> MLGTGPAAATTAATTSSNVSVLQQFASGLKSRNEETRAKAAKELQHYVTMELREMSQEESTRFYDQLNHHIFELVSSSDANERKGGILAIASLIGVEGGNATRIGRFANYLRNLLPSNDPVVMEMASKAIGRLAMAGDTFTAEYVEFEVKRALEWLGADRNEGRRHAAVLVLRELAISVPTFFFQQVQPFFDNI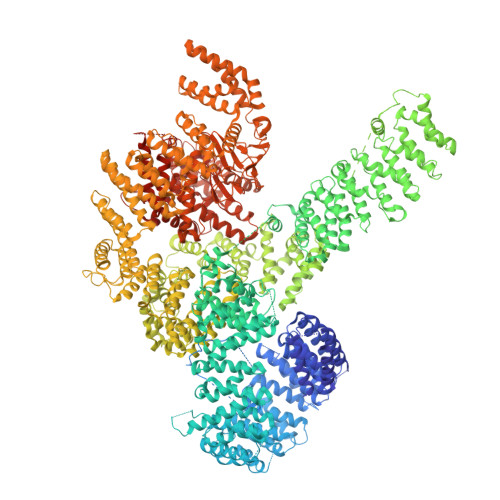FVAVWDPKQAIREGAVAALRACLILTTQREPKEMQKPQWYRHTFEEAEKGFDETLAKEKGMNRDGSTSGSGDYKDDDDKGSTSGSGDRIHGALLILNELVRISSMEGERLREEMEEITQQQLVHDKYCKDLMGFGTKPRHITPFTSFQAVQPQQSNALVGLLGYSSHQGLMGFGTSPSPAKSTLVESRCCRDLMEEKFDQVCQWVLKCRNSKNSLIQMTILNLLPRLAAFRPSAFTDTQYLQDTMNHVLSCVKKEKERTAAFQALGLLSVAVRSEFKVYLPRVLDIIRAALPPKDFAHKRQKAMQVDATVFTCISMLARAMGPGIQQDIKELLEPMLAVGLSPALTAVLYDLSRQIPQLKKDIQDGLLKMLSLVLMHKPLRHPGMPKGLAHQLASPGLTTLPEASDVGSITLALRTLGSFEFEGHSLTQFVRHCADHFLNSEHKEIRMEAARTCSRLLTPSIHLISGHAHVVSQTAVQVVADVLSKLLVVGITDPDPDIRYCVLASLDERFDAHLAQAENLQALFVALNDQVFEIRELAICTVGRLSSMNPAFVMPFLRKMLIQILTELEHSGIGRIKEQSARMLGHLVSNAPRLIRPYMEPILKALILKLKDPDPDPNPGVINNVLATIGELAQVSGLEMRKWVDELFIIIMDMLQDSSLLAKRQVALWTLGQLVASTGYVVEPYRKYPTLLEVLLNFLKTEQNQGTRREAIRVLGLLGALDPYKHKVNIGMIDQSRDASAVSLSESKSSQDSSDYSTSEMLVNMGNLPLDEFYPAVSMVALMRIFRDQSLSHHHTMVVQAITFIFKSLGLKCVQFLPQVMPTFLNVIRVCDGAIREFLFQQLGMLVSFVKSHIRPYMDEIVTLMREFWVMNTSIQSTIILLIEQIVVALGGEFKLYLPQLIPHMLRVFMHDNSPGRIVSIKLLAAIQLFGANLDDYLHLLLPPIVKLFDAPEAPLPSRKAALETVDRLTESLDFTDYASRIIHPIVRTLDQSPELRSTAMDTLSSLVFQLGKKYQIFIPMVNKVLVRHRINHQRYDVLICRIVKGYTLADEEEDPLIYQHRMLRSGQGDALASGPVETGPMKKLHVSTINLQKAWGAARRVSKDDWLEWLRRLSLELLKDSSSPSLRSCWALAQAYNPMARDLFNAAFVSCWSELNEDQQDELIRSIELALTSQDIAEVTQTLLNLAEFMEHSDKGPLPLRDDNGIVLLGERAAKCRAYAKALHYKELEFQKGPTPAILESLISINNKLQQPEAAAGVLEYAMKHFGELEIQATWYEKLHEWEDALVAYDKKMDTNKDDPELMLGRMRCLEALGEWGQLHQQCCEKWTLVNDETQAKMARMAAAAAWGLGQWDSMEEYTCMIPRDTHDGAFYRAVLALHQDLFSLAQQCIDKARDLLDAELTAMAGESYSRAYGAMVSCHMLSELEEVIQYKLVPERREIIRQIWWERLQGCQRIVEDWQKILMVRSLVVSPHEDMRTWLKYASLCGKSGRLALAHKTLVLLLGVDPSRQLDHPLPTVHPQVTYAYMKNMWKSARKIDAFQHMQHFVQTMQQQAQHAIATEDQQHKQELHKLMARCFLKLGEWQLNLQGINESTIPKVLQYYSAATEHDRSWYKAWHAWAVMNFEAVLHYKHQNQARDEKKKLRHASGANITNATTAATTAATATTTASTEGSNSESEAESTENSPTPSPLQKKVTEDLSKTLLMYTVPAVQGFFRSISLSRGNNLQDTLRVLTLWFDYGHWPDVNEALVEGVKAIQIDTWLQVIPQLIARIDTPRPLVGRLIHQLLTDIGRYHPQALIYPLTVASKSTTTARHNAANKILKNMCEHSNTLVQQAMMVSEELIRVAILWHEMWHEGLEEASRLYFGERNVKGMFEVLEPLHAMMERGPQTLKETSFNQAYGRDLMEAQEWCRKYMKSGNVKDLTQAWDLYYHVFRRISKQLPQLTSLELQYVSPKLLMCRDLELAVPGTYDPNQPIIRIQSIAPSLQVITSKQRPRKLTLMGSNGHEFVFLLKGHEDLRQDERVMQLFGLVNTLLANDPTSLRKNLSIQRYAVIPLSTNSGLIGWVPHCDTLHALIRDYREKKKILLNIEHRIMLRMAPDYDHLTLMQKVEVFEHAVNNTAGDDLAKLLWLKSPSSEVWFDRRTNYTRSLAVMSMVGYILGLGDRHPSNLMLDRLSGKILHIDFGDCFEVAMTREKFPEKIPFRLTRMLTNAMEVTGLDGNYRITCHTVMEVLREHKDSVMAVLEAFVYDPLLNWRLMDTNTKGNKRSRTRTDSYSAGQSVEILDGVELGEPAHKKTGTTVPESIHSFIGDGLVKPEALNKKAIQIINRVRDKLTGRDFSHDDTLDVPTQVELLIKQATSHENLCQCYIGWCPFW> MSTPPLAASGMAPGPFAGPQAQQAAREVNTASLCRIGQETVQDIVYRTMEIFQLLRNMQLPNGVTYHTGTYQDRLTKLQDNLRQLSVLFRKLRLVYDKCNENCGGMDPIPVEQLIPYVEEDGSKNDDRAGPPRFASEE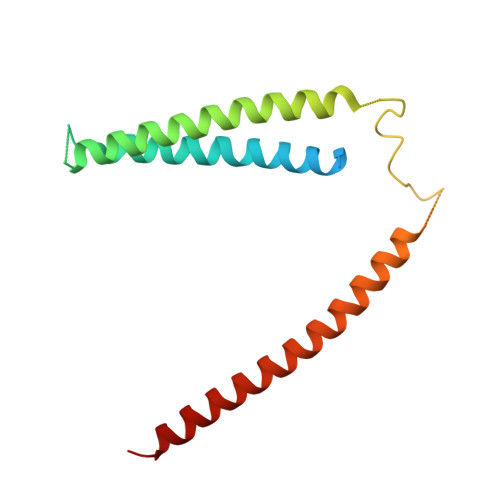RREIAEVNKKLKQKNQQLKQIMDQLRNLIWDINAMLAMRN>[5x]AMAELPPGRLATTEDYFAQQAKQAVTPDVMAQLAYMNYIDFISPFYSRGCSFEAWELKHTPQRVIKYSIAFYAYGLASVALIDPKLRALAGHDLDIAVSKMKCKRVWGDWEEDGFGTDPIEKENIMYKGHLNLMYGLYQLVTGSRRYEAEHAHLTRIIHDEIAANPFAGIVCEPDNYFVQANSVAYLSLWVYDRLHGTDYRAATRAWLDFIQKDLIDPERGAFYLSYHPESGAVKPWI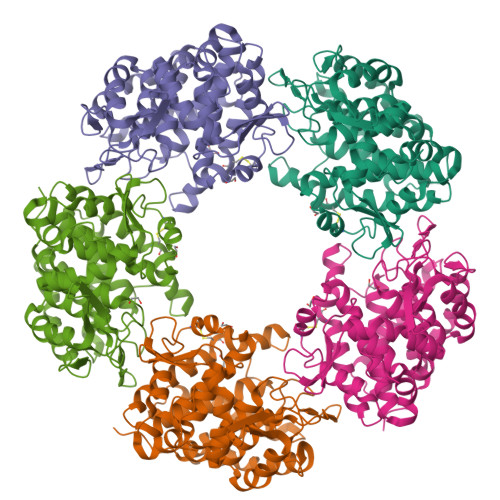SAYTTAWTLAMVHGMDPAFSERYYPRFKQTFVEVYDEGRKARVRETAGTDDADGGVGLASAFTLLLAREMGDQQLFDQLLNHLEPPAKPSIVSASLRYEHPGSLLFDELLFLAKVHAGFGALLRMPPPAAKLAGK(2S)-2-(1H-indol-3-yl)pentanoic acid | C13 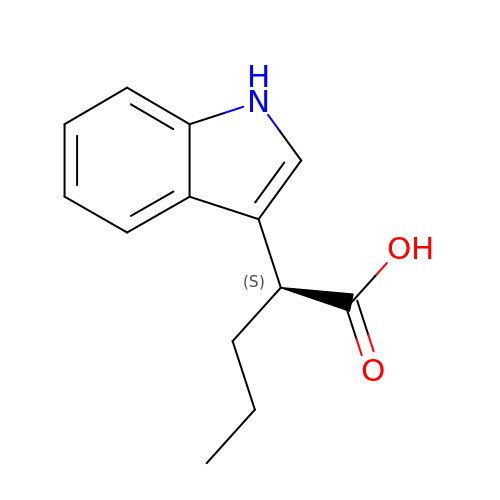H15 N O2 | QRCBLBWFQJDFJQ-JTQLQIEISA-N> SGVFQLQLQEFINERGVLASGRPCEPGCRTFFRVCLKHFQAVVSPGPCTFGTVSTPVLGTNSFAVRDDSSGGGRNPLQLPFNFTWPGTFSLIIEAWHAPGDDLRPEALPPDALISKIAIQGSLAVGQNWLLDEQTSTLTRLRYSYRVICSDNYYGDNCSRLCKKRNDHFGHYVCQPDGNLSCLPGWTGEYCQQPICLSGCHEQNGYCSKPAECLCRPGWQGRLCNECIPHNGCRHGTCSTPWQCTCDEGWGGLFCDQDLNYCTHHSPCKNGATCSNSGQRSYTCTCRPGYTGVDCELELGSHHHHHHHH

The Notch signalling pathway is conserved across all metazoan species and plays key roles in many aspects of cell biology including cell‐fate determination, stem cell maintenance, immune system activation and angiogenesis in humans (Guruharsha et al, 2012; Bray, 2016). Aberrant Notch signalling results in a number of inherited and acquired disorders, including various cancers, and it is therefore a key target for therapeutic intervention (Hansson et al, 2004; Groth & Fortini, 2012). Both the Notch receptors and the ligands are single‐pass type I transmembrane proteins, and direct protein–protein contact between adjacent cells initiates an intracellular signalling pathway. All of the Notch ligands have a modular extracellular architecture consisting of an N‐terminal C2 domain (formerly known as the MNNL domain), a Delta/Serrate/Lag‐2 (DSL) domain, and either 16 (Jagged1/Jagged2), 8 (Delta‐like1/Delta‐like4) or 7 (Delta‐like3) EGF repeats. Binding of a Notch ligand to EGF11‐12 of a Notch receptor results in a series of proteolytic cleavages, with the final intra‐membrane cleavage by gamma secretase, causing the release of the intracellular domain of Notch (NICD) from the plasma membrane.

Here, we further highlight the variability of the C2 domain putative lipid‐binding site in Notch ligands, by solving the crystal structures of N‐terminal fragments of both human Delta‐like4 and Jagged2. Here, we present the first structures of Jagged2 (N‐EGF2 and N‐EGF3), which has only 58% sequence identity with human Jagged1 (N‐EGF3), together with the longest known structure of a Delta‐like4 ligand (human Delta‐like4 N‐EGF3). For example, the angle between EGF2 and EGF3 in our hDelta‐like4 structure is likely due to interactions with a neighbouring molecule in the crystal lattice. The loops are fully ordered in Delta‐like4, and mostly ordered in Delta‐like1 (Kershaw et al, 2015) despite the absence of calcium‐binding sites in the Delta family. Consistent with this, two of the key aspartate side‐chain calcium ligands conserved in Jagged1 and 2 are replaced with arginine and histidine residues (Arg‐55 and His‐123 in Delta‐like4). The Jagged1 and Jagged2 C2 domains bind calcium ions (shown in red), whereas Delta‐like4 and Delta‐like1 do not; the aspartates involved in calcium binding are not conserved in Delta‐like4 and Delta‐like1. Even between rat and human Delta‐like4, there are loop differences, suggesting that these regions are optimized for the different mammalian physiologies (Fig EV1). There are also differences in the loops between strands 3 and 4 (CBR2), and strands 5 and 6 (CBR3) in the C2 domain between rat and human Delta‐like4 (C). A, B Delta‐like4 shows preferential binding to ganglioside‐rich liposomes compared to Jagged1 (A) whilst the converse is true for sphingomyelin‐rich liposomes (B).>[3x]MFESMKPHLAELRQRLAISVLAVFVGFIIAFTFHNAILGWITKPLNNALIQVGKIVEKREMGTWKISGNEHNATLAPSKSPALLSDHAQSAEKLHRTLAEASQATQNPKLQKLLSQAASAAEELARNSRILRKALVKEENLTRQAVNQNLREKSFNGMITTHQVGGAFFVALKVSFFAGILMAMPVILWQLWLFIAPGLYDNEKKMVLPFVVGGSVMFLIGVLFAYYVVTPFGFQFLITFGSFLYTPLINIEDYVGFFTKILIGFGIAFELPVVAYFLALLGLITDKTLKDYFKYAIVIIFLLAAFLTPPDVLTQLLMAAPLILLYGLSILIVHYVNPYKPEEKEDDEEEEEDEFEKAEREFEALEKGSESHESGSE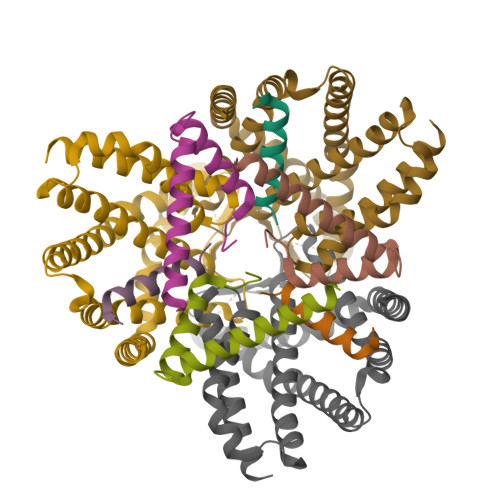NLYFQ;>[3x]MFGMGFSEILVIALVAILFLGPDKLPEAMVQIAKFFNSVRKTINEAKSTFEEELHLKELKEEALSYRQSLSEVGSDISGFKNAISNHTDELQEAIEIARSGMPTDRLNESVDDLLEEDEPTGETSQRPGVTEYKEMARKALEEAENSAEAQTAETPSVEDKGPESSPKESSRPAGFKHLDNEANAWSHPQFEK;>MQRRDFLKYSVALGVASALPLWSRAVFA[3x]3-amino-1H-isoindol-1-one 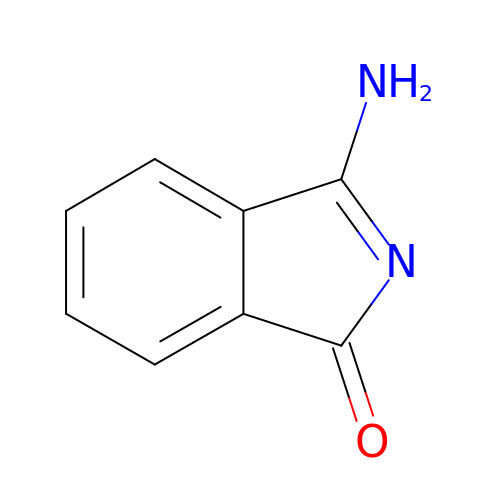| C8 H6 N2 O | MMBYJYAFFGKUDC-UHFFFAOYSA-N Eukaryotic translation initiation factor 2B (eIF2B) is the decameric guanine nucleotide exchange factor (GEF) for the GTPase eukaryotic translation initiation factor 2 (eIF2). Upon delivery of the initiator Met-tRNAi to the site of translation initiation, bound GTP is hydrolyzed and eIF2 is released from the scanning ribosome. eIF2B catalyzes GDP-GTP exchange on eIF2, enabling rebinding of Met-tRNAi to allow for a new cycle of mRNA translation initiation. Two catalytic subcomplexes, each comprised of a γ and ε subunit, decorate the central regulatory core, which is a heterohexamer composed of two α, β and δ subunits. Curiously, the eIF2B regulatory core is related to an ancient family of homo-hexameric sugar phosphate-metabolizing enzymes, with conservation observed between eIF2Bα/β/δ and the archaeal ribose-1,5-bisphosphate isomerase (RBPI).

To confirm that the binding mode for F6P is shared with other sugar phosphates, we determined the 2.7 Å crystal structure of eIF2Bα bound to M6P. Comparison of the F6P and M6P structures revealed a metabolite recognition mechanism employing the same residues in the eIF2Bα pocket. Slight differences in bonding due to the larger size of the M6P sugar could account for the difference in affinity between F6P and M6P. By contrast, the affinity of eIF2Bα for the F6P isomer mannose-6-phosphate (M6P) was considerably weaker, with Kd = 282 ± 35 μM. To identify potential changes in protein conformation upon sugar phosphate binding, we performed pairwise comparisons of eIF2B-F6P and eIF2Bα-M6P with the reported structures of apo eIF2B (PDB 7D4622) and eIF2Bα (PDB 3ECS27). eIF2Bα-M6P aligned to apo eIF2Bα with r.m.s.d. = 0.44 Å, indicating high overall similarity. Curiously, the metabolite binding site in the apo structure is occupied by SO4 molecules from the crystallization buffer. The free eIF2Bα structures also align with eIF2Bα in the context of the holoenzyme (with or without F6P) with r.m.s.d. < 0.9 Å, and interdomain orientations are not significantly changed.

>MDDKELIEYFKSQMKEDPDMASAVAAIRTLLEFLKRDKGETIQGLRANLTSAIETLCGVDSSVAVSSGGELFLRFISLASLEYSDYSKCKKIMIERGELFLRRISLSRNKIADLCHTFIKDGATILTHAYSRVVLRVLEAAVAAKKRFSVYVTESQPDLSGKKMAKALCHLNVPVTVVLDAAVGYIMEKADLVIVGAEGVVENGGIINKIGTNQMAVCAKAQNKPFYVVAESFKFVRLFPLNQQDVPDKFKYKADTLKVAQTGQDLKEEHPWVDYTAPSLITLLFTDLGVLTPSAVSDELIKLYLGGENLYFQ[8x]> QKPQRPRRPASPISTIQPKANFDAQQFAGTWLLVAVGSAARFLQEQGHRAEATTLHVAPQGTAMAVSTFRKLDGICWQVRQLYGDTGVLGRFLLQARGARGAVHVVVAETDYQSFAVLYLERAGQLSVKLYARSLPVSDSVLSGF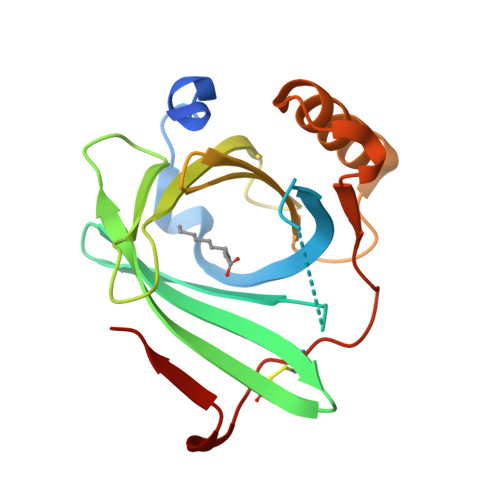EQRVQEAHLTEDQIFYFPKYGFCEAADQFHVLDEVRR>GSPEFMIGEEVPSDQYYWAPLAQHERGSLASLDSLRKGGPP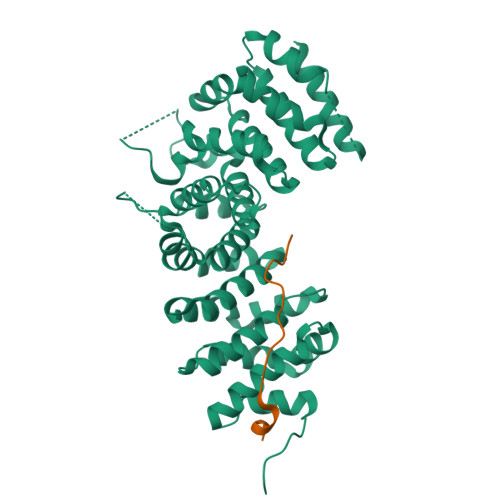PPNWRQPELPEVIAMLGFRLDAVKSNAAAYLQHLCYRNDKVKTDVRKLKGIPVLVGLLDHPKKEVHLGACGALKNISFGRDQDNKIAIKNCDGVPALVRLLRKARDMDLTEVITGTLWNLSSHDSIKMEIVDHALHALTDEVIIPHSGWEREPNEDCKPRHIEWESVLTNTAGCLRNVSSERSEARRKLRECDGLVDALIFIVQAEIGQKDSDSKLVENCVCLLRNLSYQVHREIPQAERYQEAAPNVANNTGTSPARGYELLFQPEVVRIYISLLKESKTPAILEASAGAIQNLCAGRWTYGRYIRSALRQEKALSAIADLLTNEHERVVKAASGALRNLAVDARNKELIGKHAIPNLVKNLPGGQQNSSWNFSEDTVISILNTINEVIAENLEAAKKLRETQGIEKLVLINKSGNRSEKEVRAAALVLQTIWGYKELRKPLEKEGWKKSDFQVNLNNASRSQSSHSYDDSTLPLIDRNQKSDKKPDREEIQMSNMGSNTKSLDNNYSTPNERGDHNRTLDRSGDLGDMEPLKGTTPLMQKI[3x];>DEEGGGEEDQDFDLSQLH[3x]>MASMKKKGSVVIVGRINLSGDTAYAQQTRGEEGCQETSQTGRDKNQVEGEVQIVSTATQTFLATSINGVLWTVHHGAGTRTIASPKGPVTQMYTNVDKDLV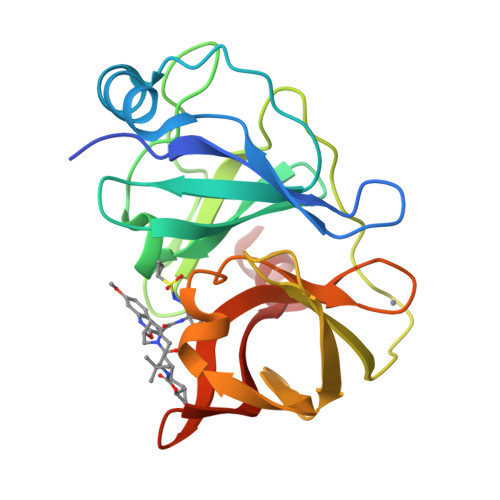GWQAPQGSRSLTPCTCGSSDLYLVTRHADVIPVRRRGDSRGSLLSPRPISYLKGSSGGPLLCPAGHAVGIFRAAVSTRGVAKAVDFIPVESLETTM[4x]>AKYYNEPCHTFNEYLLIPGLSTVDCIPSNVNLSTPLVKFQKGQQSEINLKIPLVSAIMQSVSGEKMAIALAREGGISFIFGSQSIESQAAMVHAVKNFKDSQKRYLVGAGINTRDFRERVPALVEAGADVLCIDSSDGFSEWQKITIGWIRDKYGDKVKVGAGNIVDGEGFRYLADAGADFIKIGIGGGSICITREQKGIGRGQATAVIDVVAERNKYFEETGIYIPVCSDGGIVYDYHMTLALAMGADFIMLGRYFARFEESPTRKVTINGSVMKEYWGEGSSRARNWQRYDLGGKQKLSFEEGVDSYVPYAGKLKDNVEASLNKVKSTMCNCGALTIPQLQS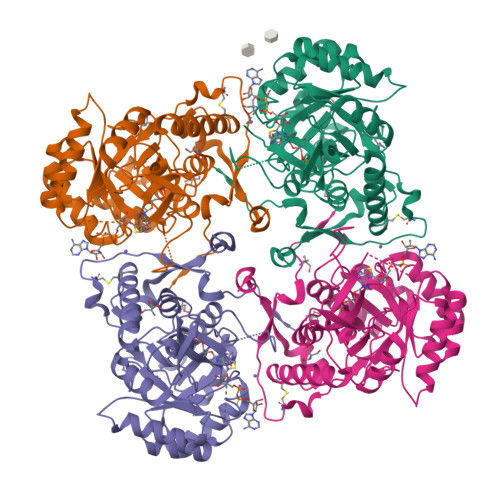KAKITLVSSVSIVEGGAHDVIVKDRINDYHPK[4x]>VLYRAVQLLILLYFVWYVFIVQKSYQESETGPESSIITKVKGITTSEHKVWDVEEYVKPPEGGSVFSIITRVEATHSQTQGTCPESIRVHNATCLSDADCVAGELDMLGNGLRTGRCVPYYQGPSKTCEVFGWCPVEDGASVSQFLGTMAPNFTILIKNSIHYPKFHFSKGNIADRTDGYLKRCTFHEASDLYCPIFKLGFIVEKAGESFTELAHKGGVIGVIINWDCDLDLPASECNPKYSFRRLDPKHVPASSGYNFRFAKYYKINGTTTRTLIKAYGIRIDVIVHGQAGKFSLIPTIINLATALTSVGVGSFLCDW[3x]

The P2X2 receptor (P2X2R) is an adenosine triphosphate (ATP)-gated ion channel with few small-molecule modulators that exhibit poor pharmacological properties. It is known to be involved in the auditory system and has been proposed as a drug target for age- and noise-related hearing loss. Each P2X2 protomer is composed of intracellular N and C termini and two transmembrane (TM) helices (outer TM1 and pore-lining TM2) connected by a voluminous extracellular domain. Three P2X2 protomers intertwine to form the trimeric receptor, with each subunit adopting a dolphin-like shape, as first established for the zebrafish P2X4R (zfP2X4R).

Using cryo-EM we determined two distinct structures (obtained from two different purification approaches) with ATP bound in the orthosteric binding sites and a uniquely constricted pore, consistent with desensitized state conformations. Both desensitized state structures, which we refer to as conformation I and conformation II, were determined at high resolution (2.5 Å, and 2.6 Å, respectively). In conformation II, the left flipper (residues 288–299) adopts an alternate pose compared to conformation I, abrogating an interaction with ATP. In contrast, in conformation II, the loop containing S296 is flipped away from the orthosteric pocket, resulting in S296 pointing in the opposite direction, now at a distance of 8.0 Å from the α-phosphate of ATP. As a result of this alternate conformation, there is one less interaction with ATP and a larger opening to the ATP-binding pocket. During cryo-EM data processing from the second purification, we were able to classify two distinct conformational states; the apo closed state conformation in addition to the alternate ATP-bound desensitized state conformation II, which has not been described before. We speculate that the adjusted purification conditions (depletion of ATP using apyrase and addition of Ca2+-ions) allowed us to capture both conformations. Finally, when conformation II was used for MD simulations, the left flipper starts in an “open pocket” conformation, with an initial distance between S296 and the α-phosphate of ATP of 8.0 Å. The left flipper of conformation II was also mobile during the simulations moving between distances above and below 4.0 Å for the aforementioned interaction (S19 D–F). Thus, we speculate that conformation II captures the receptor in a transitionary state where the movement of the loop might facilitate release of ATP from the orthosteric pocket in the desensitized state of hP2X2R.> GDRVADVIESSIGDSVSRALTRALPAPTGQDTQVSSHRLDTGKVPALQAAEIGASSNASDESMIETRCVLNSHSTAETTLDSFFSRAGLVGEIDLPLEGTTNPNGYANWDIDITGYAQMRRKVELFTYMRFDAEFTFVACTPTGQVVPQLLQYMFVPPGAPKPDSRESLAWQTATNPSVFVKLSDPPAQVSVPFMSPASAY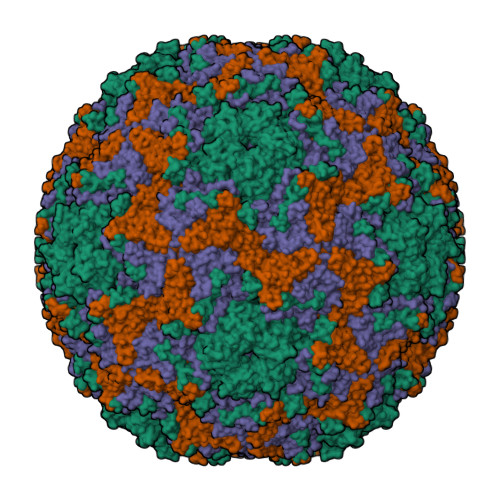QWFYDGYPTFGEHKQEKDLEYGACPNNMMGTFSVRTVGTSKSKYPLVIRIYMRMKHVRAWIPRPMRNQNYLFKANPNYAGNFIKPTGASRTAITTL;> SPSAEACGYSDRVAQLTIGNSTITTQEAANIIVGYGEWPSYCSDSDATAVDKPTRPDVSVNRFYTLDTKLWEKSSKGWYWKFPDVLTETGVFGQNAQFHYLYRSGFCIHVQCNASKFHQGALLVAVLPEYVIGSVAGGTGTEDTHPPYKQTQPGADGFELQHPYVLDAGIPISQLTVCPHQWINLRTNNCATIIVPYINALPFDSALNHCNFGLLVVPISPLDYDQGATPVIPITITLAPMCSEFAGLRQAVTQ;> GFPTELKPGTNQFLTTDDGVSAPILPNFHPTPCIHIPGEVRNLLELCQVETILEVNNVPTNATSLMERLRFPVSAQAGKGELCAVFRADPGRSGPWQSTLLGQLCGYYTQWSGSLEVTFMFTGSFMATGKMLIAYTPPGGPLPKDRATAMLGTHVIWDFGLQSSVTLVIPWISNTHYRAHARDGVFDYYTTGLVSIWYQTNYVVPIGAPNTAYIIALAAAQKNFTMKLCKDASDILQTGTIQ;> MGSQVSTQRSGSHENSNSATEGSTINYTTINYYKDSYAATAGKQSLKQDPDKFANPVKDIFTEMAAPLK> MEAYITEMVSRERANELEVYVYVFPRKQSDNNYEGVYHIMRAWQRANDLPLAYNQHTIMAFSPVRHMCGYTPMETQKRHINIDSPFERALLERLIKNSLIFTAERHLHAKRVGHALRLNQVQQIRQVIIYEAIELYVNIIENRISIGFHLTHQFEYVYTLQSMIEQGKTIRPGMRVVHSNGRQHYTYTVENVATYGVTDRCPLLQTSIYQYYVEKGAQHILRTFTRSTRVIHVRTKEQRLSYAATLLKPLCTFETMQPQDVLNVSKCIKLSASKRMKCTYRWIQQLRAQYRHLTFAPNPFTIAQNGYKLDQLSTPKVHFHRDYATVVSGMKTGKLYKGGNIKISVLFDEDFYLKHHITKKDIYQFIAVLQKIAIAQGVNMTISTSTKSITGKFTDDFFHHFTEEVEALQPIFAQTTVLAFITSTHLSNKKTRSYQLLKQYFGGKWDIASQVITEKTIEAFQKILHKHGLKNFYPNDEQHCLRVIDVLKNESFYYTVMNILLGVYVKSGIQPWILANTTHSDCFIGIDVSHENGNSAAGMMNVIGSQGHLIQQAPLNGILAGEKIDDTLLANLLKQMIKAYHTQFQRFPKHITIHRDGFWREHTALVEKIMSHYEITYDIVEIIKKPNRRMAFFNSVDNTFSTRQGTVYQRG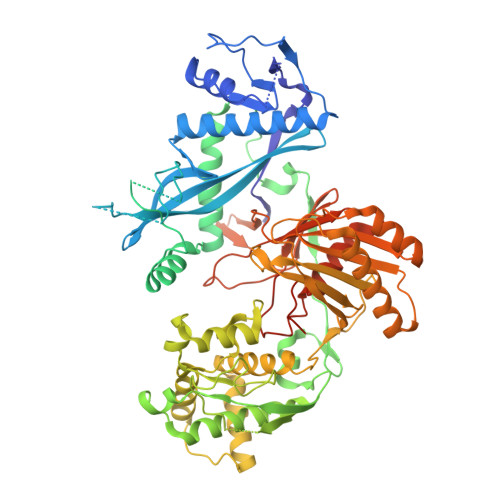NEAFLCATNPQQKVGMAQPIKIHQVTKTLPFSHIIEDVYNLSFLHIHAMNKMRLPATIHYADLSATAYQRGQVMPRSGNQTNLPFV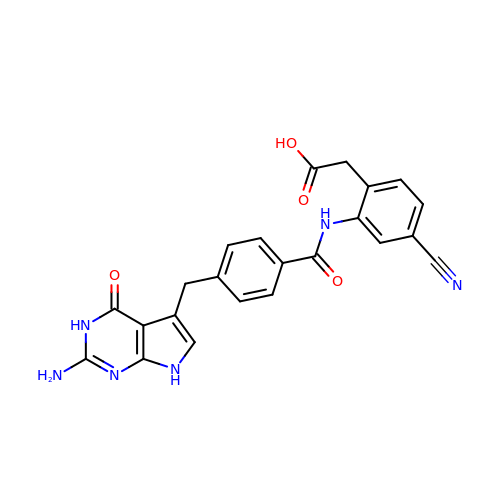[2-({4-[(2-amino-4-oxo-4,7-dihydro-3H-pyrrolo[2,3-d]pyrimidin-5-yl)methyl]benzene-1-carbonyl}amino)-4-cyanophenyl]acetic acid | C23 H18 N6 O4 | ZVNRPTCYZJBJNB-UHFFFAOYSA-N> SGSGRIIYDR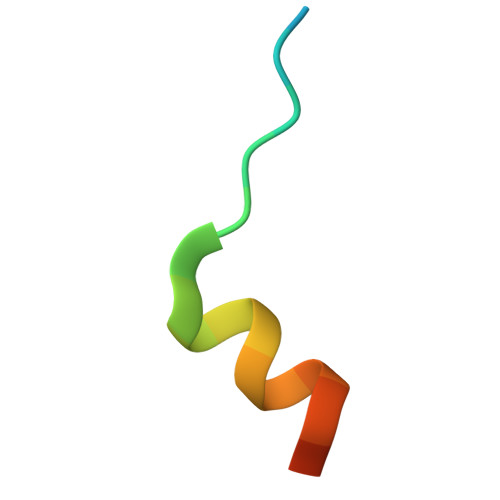KFLMECRNSPV>GAMSCVYAFGSNGQRQLGLGHDEDMDTPQRSVPGDDGAIVRKIACGGNHSVMLTNDGNLVGCGDNRRGELDSAQALRQVHDWRPVEVPAPVVDVACGWDTTVIVDADGRVWQRGGGCYEFTQQHVPLNSNDERIAVYGCFQNFVVVQGTRVYGWGSNTKCQLQEPKSRSLKEPVLVYDTGSVAVDYVAMGKDFMVIVDEGGRIVHASGRLPTGFELKQQQKRHNLVVLCMWTSIHLWNARLNTVESFGRGTHSQLFPQERLDFPIVGVATGSEHGILTTANQEGKSHCYNVYCWGWGEHGNCGPQKGSQPGLQLVGQYSGKPRVFGGCATTWIVLGSGSGSGSGSMSTYDEIEIEDMTFEPENQMFTYPCP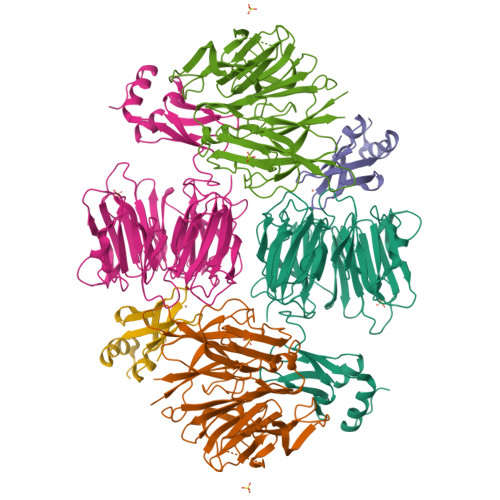CGDRFQIYLDDMFEGEKVAVCPSCSLMIDVVFDKEDLAEYYEEAGIHPPEPIAAAA[3x]>[2x]MKETAAAKFERQHMDSS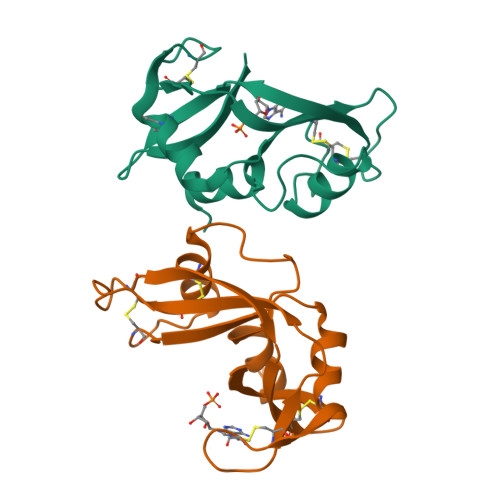TSAASSSNYCNQMMKSRNLTKDRCKPVNTFVHESLADVQAVCSQKNVACKNGQTNCYQSYSTMSITDCRETGSSKYPNCAYKTTQANKHIIVGCEGNPYVPVHFDASV>MSIKIRDFGLGSDLISLTNKAGVTISFTNLGARIVDWQKDGKHLILGFDSAKEYLEKDAYPGATVGPTAGRIKDGLVKISGKDYILNQNEGPQTLNGGEESIHTKLWTYEVTDLGAEVQVKFSLVSNDGTNGYPGKIEMSVTHSFDDDNKWKIHYEAISDKDTVFNPTGHVYFNLNGDASESVENHGLRLAASRFVPLKDQTEIVRGDIVDIKNTDLDFRQEKQLSNAFNSNMEQVQLVKGIDHPFLLDQLGLDKEQARLTLDDTSISVFTDQPS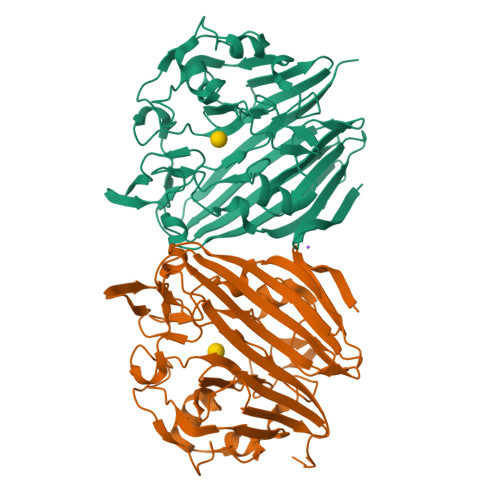IVIFTANFGDLGTLYHEKKQVHHGGITFECQVSPGSEQIPELGDISLKAGEKYQATTIYSLHTKLEHHHHHH[2x]> SNAMNILIIGNGGREHALGWKAAQSPLADKIYVAPGNAGTALEPTLENVDIAATDIAGLLAFAQSHDIGLTIVGPEAPLVIGVVDAFRAAGLAIFGPTQAAAQLEGSKAFTKDFLARHNIPSAEYQNFTDVEAALAYVRQKGAPIVIKADGLAAGKGVIVAMTQEEAETAVNDMLAGNAFGDAGHRIVVEEFLDGEEASFIVMVDGENVLPMATSQDHKRVGDGDTGPNTGGMGAYSPAPVVTDDVHQRVMDQVIWPTVRGMAAEGNIYTGFLYAGLMISADGQPKVIEFNCRFGDPETQPIMLRMRSDLVELCLAGTQGKLNEKTSDWDERPSLGVVLAAGGYPADYRQGDVIHGLPQQEVKDGKVFHAGTKLNGNH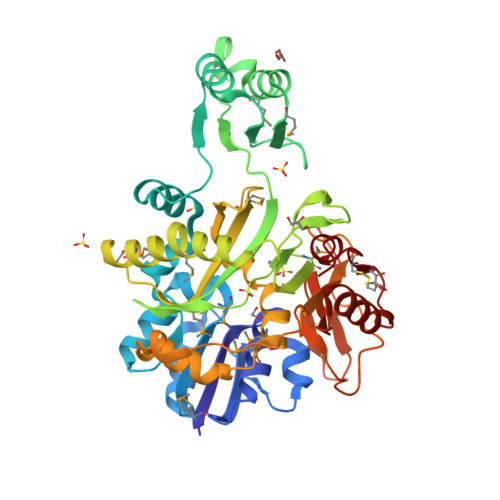EVVTNGGRVLCVTALGETVAQAQQYAYQLAEGIQWEGVFCRKDIGYRAIARGK>[16x]MRKKSLTIFSDGTLLRRE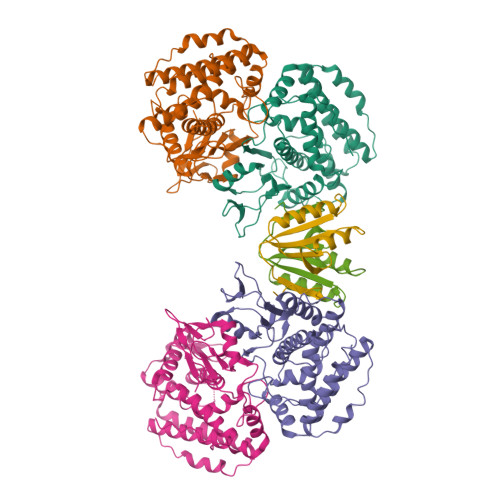NTLYFENVNGRKPLAIEGIYDIYIYGHVNITSQALHYIAQKGILIHFFNHYGYYDGTFYPRETLLSGDLIIKQAEHYLDKNKRLFLAKSFVVGGAKNMEKNLKNWGISSDFSNHLKELQGAKKVTEIMNVEGRIRQEYYARWDESLPGEFRIGKRTRRPPKNEMNALISFLNSRLYATMISEIYNTQLAPTISYLHEPSERRFSLALDLSEIFKPIIADRIANRLVKKGIIKKDHFREDLNGVLLTDEGMKIVTKAYNQELEKTVKHPKLGKGVTRRRLIRLEAYKIIKHLVGVEEYSPLVAWF;>MYIVVVYDVGVERVNKVKKFLRMHLNWVQNSVFEGEVTLAEFERIKEGLKKIIDENSDSVIIYKLRSMPPRETLGIEKNPIEEII[8x]>[2x]MTTQTTPAHIAMFSIAAHGHVNPSLEVIRELVARGHRVTYAIPPVFADKVAATGARPVLYHSTLPGPDADPEAWGSTLLDNVEPFLNDAIQALPQLADAYADDIPDLVLHDITSYPARVLARRWGVPAVSLSPNLVAWKGYEEEVAEPMWREPRQTERGRAYYARFEAWLKENGITEHPDTFASHPPRSLVLIPKALQPHADRVDEDVYTFVGACQGDRAEEGGWQRP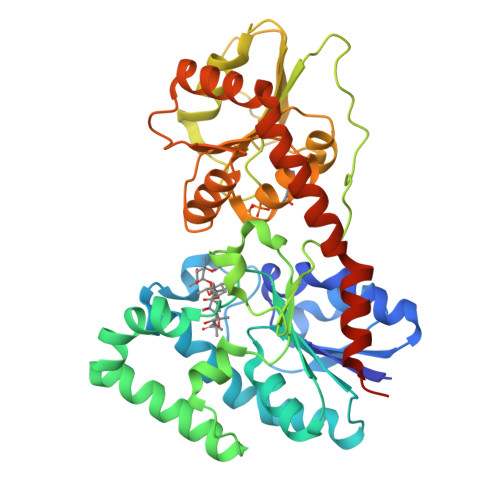AGAEKVVLVSLGSAFTKQPAFYRECVRAFGNLPGWHLVLQIGRKVTPAELGELPDNVEVHDWVPQLAILRQADLFVTHAGAGGSQEGLATATPMIAVPQAVDQFGNADMLQGLGVARKLATEEATADLLRETALALVDDPEVARRLRRIQAEMAQEGGTRRAADLIEAELPARHERQEPVGDRPNGG>[2x]SVDREEMIERFANFLREYTDEDGNPVYRGKI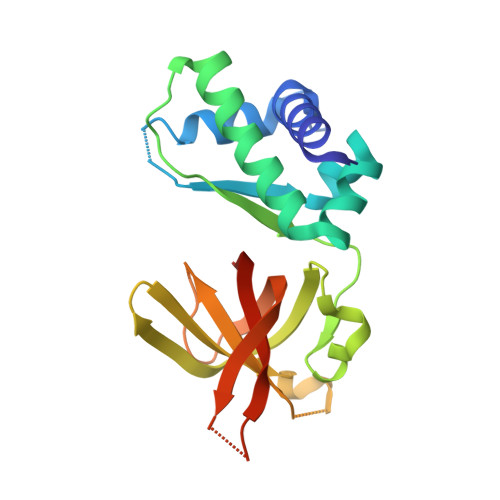TDLLTITPKRSVAIDWMHLNSFDSELAHEVIENPEEGISAAEDAIQIVLREDFQREDVGKIHARFYNLPETLMVKDIGAEHINKLIQVEGIVTRVGEIKPFQSFRIQDRPETLKGGEMPRFIDGILLDDIVDVALPGDRVIVTGILRVVLEKREKTPIFRKILEVNHIEPVSKEI>MHHH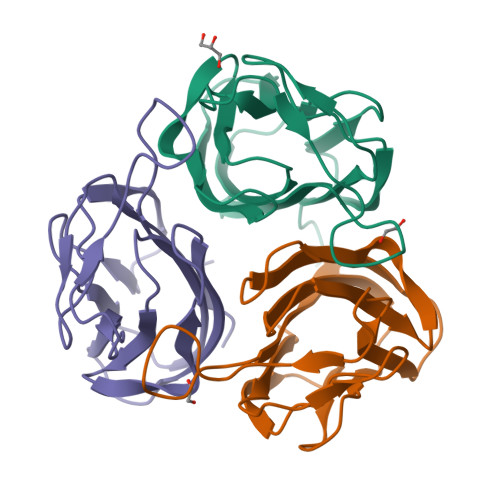HHHSVGLTNYLYVFDTTNQSIAVGSSVTFNTNGPITGTALSHITGTGNIIINTLGTYVAEFQLQASRENQFSLELNGTPIPGGRFGTGSPHSINQGTAAFTVTVVPSTLTLINNTSSAGTITLSNSDGGSLTNVSASISIFQVG[21x]>[6x]MGKVYKKVELVGTSEEGLEAAIQAALARARKTLRHLDWFEVKEIRGTIGEAGV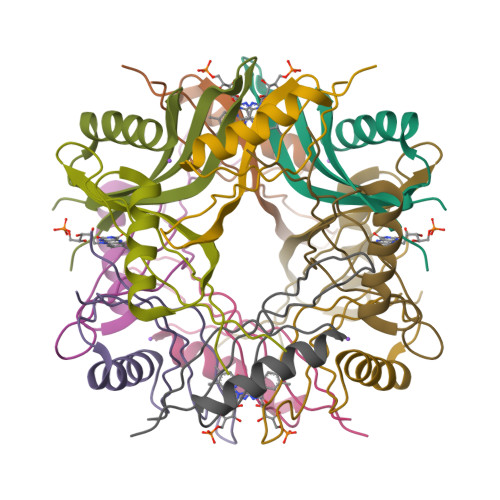KEYQVVLEVGFRLEET> MKKGHHHHHHENLYFQGGSAPG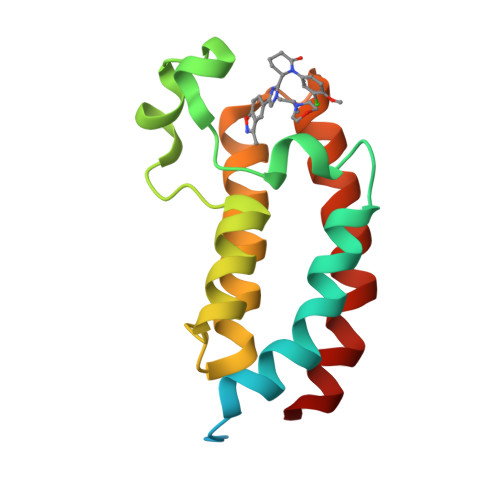QSKKKIFKPEELRQALMPTLEALYRQDPESLPFRQPVDPQLLGIPDYFDIVKSPMDLSTIKRKLDTGQYQEPWQYVDDIWLMFNNAWLYNRKTSRVYKYCSKLSEVFEQEIDPVMQSLG> GEEEKKRTARTDYWLQPEIIVKIITKKLGEKYHKKKAIVKEVIDKYTAVVKMIDSGDKLKLDQTHLETVIPAPGKRILVLNGGYRGNEGTLESINEKTFSATIVIET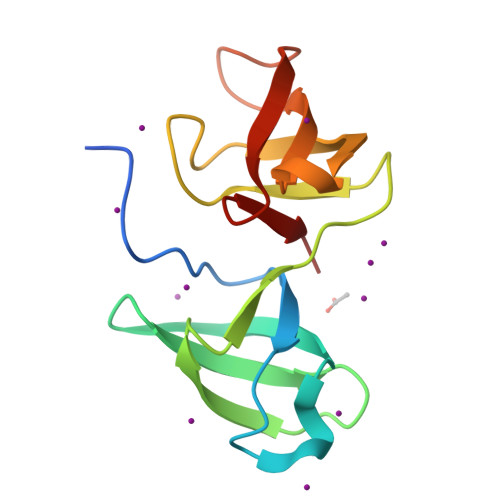GPLKGRRVEGIQYEDISKLA>GFFSFIGEAFQGAGDMWRAYTDMKEAGWKDGDKYFHARGNYDAAQRGPGGVWAAEKISDARESFQEFFGRGHEDTMADQEANRHGRSGKDPNYYRPPGLPAKY[12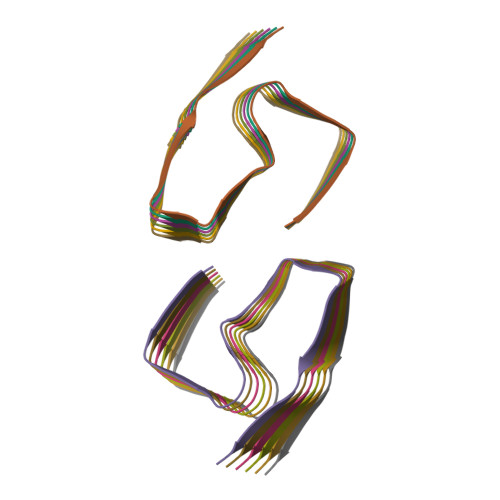x]>GSHMQDPEQLKHCNGILKELLSKKHAAYAWPFYKPVDASALGLHDYHDIIKHPMDLSTVKRKMENRDYRDAQEFAADVRLMFSNCYKYNPPDHDVVAMARKLQDVFEFRY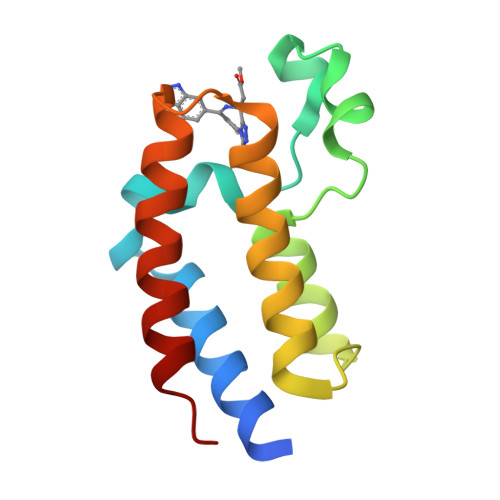AKMPD[2x]>GPMADPWQECMDYAVTLARQAGEVVCEAIKNEMNVMLKSSPVDLVTATDQKVEKMLISSIKEKYPSHSFIGEESVAAGEKSILTDNPTWIIDPIDGTTNFVHRFPFVAVSIGFAVNKKIEFGVVYSCVEGKMYTARKGKGAFCNGQKLQVSQQEDITKSLLVTELGSSRTPETVRMVLSNMEKLFCIPVHGIRSVGTAAVNMCLVATGGADAYYEMGIHCWDVAGAGIIVTEAGGVLMDVTGGPFDLMSRRVIAANNRILAERIAKEIQVIPLQRDDED[2x]

IMPase is a key enzyme in the intracellular phosphatidyl­inositol (PI) signalling pathway, whereby IMPase dephos­phorylates inositol 1-, 3- or 4-phosphate, collectively known as InsP1, to produce myo-inositol, also known as free inositol. Cleavage of InsP1 into myo-inositol by IMPase is required for the recycling of inositol for subsequent use in the PI signalling pathway. One enzyme inhibited by lithium is inositol monophos­phatase (IMPase; Gill et al., 2005), which has led to rational drug design targeting IMPase as a strategy for developing novel therapies for bipolar disorder. One such IMPase inhibitor is ebselen [2-phenyl-1,2-benz­isoselenazol-3(2H)-one], an organoselenium compound which functions as a glutathione peroxidase mimic.

In this structure, ebselen is in an open-ring conformation, with the Se atom forming a selenosulfide bond to the sulfur group of Cys141, which is consistent with the known binding mechanism of ebselen. IMPase contains seven cysteine residues, amino acids 8, 24, 125, 141, 184, 201 and 218; of these residues, only Cys218 is near the active site. IMPase is a dimeric enzyme and in the crystal structure two adjacent dimers share four ebselen molecules, creating a tetramer with approximate 222 symmetry. The binding of ebselen to the Cys141 residue in each monomer does not lead to noticeable changes in conformation in the active site that would prevent the catalytic activity of IMPase. In the crystal structure presented in this publication, the active site in the tetramer is still accessible, suggesting that ebselen may function as an allosteric inhibitor or may block the binding of partner proteins. Previous research suggested that Cys218 is the primary reactive cysteine residue, which is supported by the reduced inhibition of C218A mutant IMPase by ebselen. However, whilst this structure clearly shows ebselen bound to Cys141 in each monomer of IMPase, our structure does not rule out the possibility that Cys218 could be modified in vivo. There is evidence that modulation of IMPase away from the active site and dimer interface can affect activity; synthetic peptides that disrupt IMPase–calbindin interactions prevent calbindin-mediated activation of IMPase and mediate antidepressant-like effects in mice. It is possible that ebselen interferes with accessory protein binding, possibly by formation of the tetramer seen in the crystal, to moderate the activity of IMPase in vivo.> MVALSLKISIGNVVKTMQFEPSTMVYDACRMIRERIPEALAGPPNDFGLFLSDDDPKKGIWLEAGKALDYYMLRNGDTMEYRKKQRPLKIRMLDGTVKTIMVDDSKTVTDMLMTICARIGITNHDEYSLVRELMEEKKDDELNWLDHGRTLREQGVEEHETLLLRRKFFYSDQNVDSRDPVQLNLLYVQARDDILNGSHPVSFDKACEFAGFQCQIQFGPHNEQKHKAGFLDLKDFLPKEYVKQKGERKIFQAHKNCGQMSEIEAKVRYVKLARSLKTYGVSFFLVKEKMKGKNKLVPRLLGITKECVMRVDEKTKEVIQEWSLTNIKRWAASPKSFTLDFGDYQDGYYSVQTTEGEQIAQLIAGYIDIIL

The FERM domain protein talin (∼270 kDa) plays a key role in activation of the integrin family of cell adhesion receptors and also provides a direct link between the cytoplasmic tail of the β-integrin subunit and the actin cytoskeleton. Talin consists of a ∼50 kDa N-terminal head and an elongated 220 kDa rod composed of amphipathic helical bundles. The talin head contains a FERM domain which is similar to that found in ERM proteins, although it has two novel features: the F1 domain includes a 30 residue unstructured loop and is preceded by an additional domain (F0) which, like F1, has a ubiquitin-like fold (Goult et al., 2010). The integrin binding site is located in the F3 domain and, although a second integrin binding site exists within the talin rod (Gingras et al., 2009), only constructs containing the F3 domain are able to activate integrins (Calderwood et al., 2002).

We also established that the talin head contains an additional globular domain F0 at the N terminus that is closely associated with the F1 domain (Goult et al., 2010). Based on these results, we extended the FERM domain construct to include F0 (residues 1–400) and removed the unstructured F1 loop (residues 139–168), as illustrated in Figure 1A. Overall, the model contains 358 residues and 561 solvent molecules with an average B factor of 18 Å2 (overall) and 25 Å2, respectively. One molecule was observed within the asymmetric unit and is shown in Figure 1B. The structure of TH′ consists of four domains arranged in a novel linear configuration. Both F0 and F1 domains have ubiquitin-like folds, the F2 domain contains a core 4-helix bundle equivalent to that found in acyl-CoA-binding protein, and the F3 domain has a phosphotyrosine binding domain (PTB) fold. The interfaces F0-F1 and F2-F3 each form a network of close contacts that stabilize the relative domain orientations. In contrast, despite a similar buried surface area of 620 Å2, the F1-F2 interface is loosely packed with no specific interactions apart from a single hydrogen bond between the carbonyl of Q288 and the guanidinium group of R194. The F1-F2 linker region in talin (residues 196–208) adopts a distinctly different β-hairpin-like conformation in the F198-S205 region. The packing of the linker region against F2 positions the F1 domain on the opposite surface of F2 relative to F3. The location of all the membrane-binding residues on the same face of the talin head indicates that they can all simultaneously associate with the membrane, thus generating high affinity binding through multiple dispersed interactions.As such, we found that a circularly permuted variant of a cage-forming enzyme, Aquifex aeolicus lumazine synthase, cpAaLS, assembles into a variety of hollow spherical and cylindrical structures in response to changes in ionic strength. Cryogenic electron microscopy revealed that these structures are composed entirely of pentameric subunits, and the dramatic cage-to-tube transformation is attributed to the moderately hindered 3-fold symmetry interaction and the imparted torsion angle of the building blocks, where both mechanisms are mediated by an α-helix domain that is untethered from the native position by circular permutation. While the wild-type protein, AaLS-wt, self-assembles into a ∼ 16 nm dodecahedral structure composed of 60 identical monomers,35 the negatively supercharged variants AaLS-neg and AaLS-13 adopt expanded 360- and 720-mer assemblies, respectively, constructed entirely from pentameric capsomers. Moreover, a circularly permuted variant of AaLS, cpAaLS(119), forms not only ∼24 nm and ∼28 nm expanded spherical cages, but also straight ∼24 nm-wide tubes of variable length. We previously designed two circularly permuted variants of AaLS and confirmed that their morphologies depend on the positions of the newly generated N- and C-termini. The native terminal amino acids were connected via an octapeptide linker using genetic fusion and new sequence termini were introduced either between residues 84 and 85 or 119 and 120, yielding cpAaLS(84) or cpAaLS(119), respectively.

The cpAaLS(84) assembly resembles the AaLS-wt cage, where each pentamer interacts with five neighboring subunits in a dodecahedral arrangement. The atomic model of the cpAaLS(84) cage revealed that all the constituent pentamers interact with each other in the same manner as in the AaLS-wt assembly. The 2-fold symmetry interface consists of a hydrophobic patch (L8, L141, and W137) surrounded by a hydrogen bond (H41) and ionic interactions (e.g., R40 and E5) while an α-helix region (120–131) forms 3-fold symmetric hydrophobic clusters (I121 and I125) in the cage interior. Irrespective of the tested buffer conditions, cpAaLS(84) did not exhibit substantial fluorescent changes up to 110 °C, indicating little protein unfolding.

>[60x]MATPHFDYIASEVSKGLANLSLELRKPITFGVITADTLEQAIERAGTKHGNKGWEAALSAIEMANLFKSLRGTGGSGSSMEIYEGKLTAEGLRFGIVASRFNHALVDRLVEGAIDCIVRHGGREEDITLVRVPGSWEIPVAAGELARKEDIDAVIAIGVLIRG> SNAMVTLYTTKYCPYSLRARIALAEKK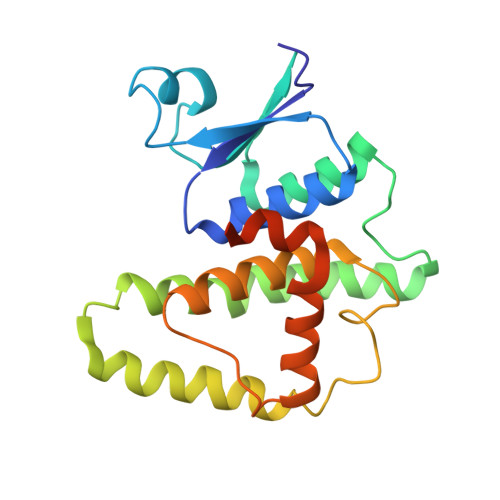MSTDIVEAGDLEPAMIKKITPNGVFPVLMEKDYSINNRKALLIYIDERFPAPSLLPNVVNERIKIRLSLDKIDNEWYPVLDQIRKHRSDQKMLESMFKDLKESLLAMEKAFTGSEFFISSGFTLADCYIAALIICLEAEGFIIDDEYGAIYEYKKRLFARDSVKKANIKGGAGESLLKTLRTHR>GMTDRLKGKVAIVTGGT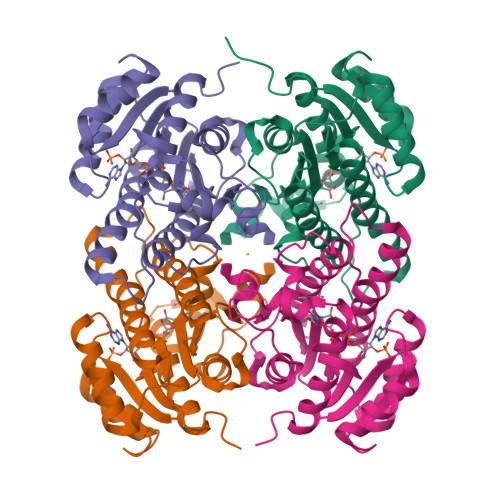LGIGLAIADKFVEEGAKVVITGRHADVGEKAAKSIGGTDVIRFVQHDASDEAGWTKLFDTTEEAFGPVTTVVNNAGIAVSKSVEDTTTEEWRKLLSVNLDGVFFGTRLGIQRMKNKGLGASIINMSSIEGLVGDPTQGAYNASKGAVRIMSKSAALDCALKDYDVRVNTVHPGPIKTPLVDDAEGAEEFFSQRTKTPMGHIGEPNDIAWICVYLASDESKFATGAEFVVDGGYTAQ[4x]>[4x]EYGYIVTDQKPLSLAAGVKLLEILAEHVHMSSGSFINISVVGPALTFRIR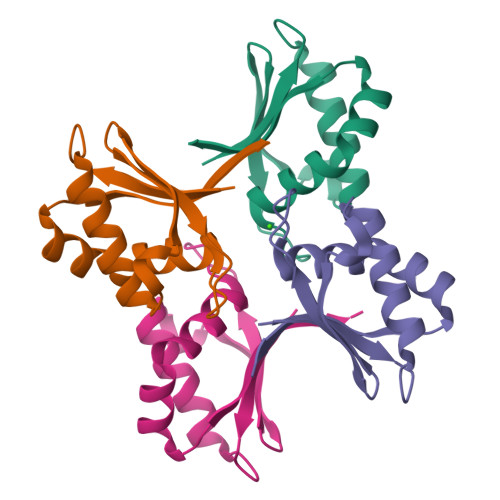HNEQNLSLADVTQQAGLVKSELEAQTGLQILQTGVGQRE>[2x]TNRDIQFTSFNGKDYPLCFLDEKTPLLFQWFERNPARFGKNDIPIINTEKNPYLNNIIKAATIEKERLIGIFVDGDFFPGQKDAFSKLEYDYENIKVIYRNDIDFSMYDKKLSEIYMENISKQESMPEEKRDCHLLQLLKKELSDIQEGNDSLIKSYLLDKGHGWADFYRNMAMLKAGQLFLEADKVGCYDLSTNSGCIYLDADMIITEKLGGIYIPDGIAVHVERIDGRASMENGIIAVDRNNHPALLAGLEIMHTKFDADPYSDGVCNGIRKHFNYSLNEDYNSFCDFIEFKHDNIIMNTSQ

Escherichia coli NleB1, Citrobacter rodentium NleB, and Salmonella enterica SseK1/3 type III effectors fatally glycosyltransfer N-acetyl glucosamine (GlcNAc) from UDP-GlcNAc to arginine residues of death domain-containing proteins that regulate host inflammation, intra-bacterial proteins, and themselves, whose post-translational modification disrupts host immune functions and prolongs bacterial viability inside host cells. All NleB/SseK orthologs have a typical GT-A conformation with two abutting β/α/β Rossmann domains unlike a GT-B consisting of facing each other β/α/β Rossmann domains with a flexible linkage and share a high degree of structural similarity. Several structural cores were revealed for the new arginine N-glycosylation systems: a catalytic DxD motif to position the Mn2+ cofactor and UDP-GlcNAc donor substrate, His-Glu-Asn (HEN) motif to select UDP-GlcNAc as a suitable donor substrate before other sugar donors such as UDP-Glc/Gal, C-terminal loop to stably embrace the UDP-GlcNAc donor substrate, and Helix-Loop-Helix (HLH) domain predicted to select the acceptor targets. The SseK1 effector GlcNAcylates Arg9, Arg190, Arg160, and Arg149 of four proteins involved in methylglyoxal detoxification, namely, GloA, GloB, GloC, and YajL, respectively, and catalyze methylglyoxal detoxification to significantly enhance their activity.

In all apo- and UDP-bound NleB1/SseK1/SseK3 effectors, the DxD motifs lie in the 219YLDADM224/221YLDADM226/224YLDADM229 regions and their quaternary DADM motifs form a Type-I-turn by H-bonding between the backbone CO(i) and NH(i + 3) groups, while the free Asp oxygen (Oδ of Asp221/Asp223/Asp/226) in the DxD motif interacts with the hydroxyl oxygen (Oη of Tyr219/Tyr221/Tyr224), named as a YD bond. In particular, apo NleB1/SseK1/SseK3 effectors have the free oxygen Oδ of the first catalytic aspartate in the DxD motif, ready to catch Mn2+ and UDP-GlcNAc. All N-glycosylated NleB/SseKs form a Type-I-turn in the DxD motif in the ligand-bound state, and the pathogenic NleB1/SseK1/3 toxins also retain Type-I-turn in the DxD motif in the apo state. Apo Clostridium toxin TcnA and apo E. coli NleB2 have twice intertwined Asx-β-turns, where Type-I-turns H-bond between the backbone CO of D284/D218 and the backbone NH of F287/M221, and the Asx-turn C10 H-bonds between the side chain of D284/D218 and NH of D286/D220 in apo TcnA/NleB2. These results indicate that the first catalytic aspartate in Apo TcdA/B, TcsL, SseK1/3, and NleB1 DxD motifs is open to bind Mn2+, whereas those of Apo TcnA, SseK2, and NleB2 are tightly tied by the second aspartate backbone in the Asx-turn of the DxD motif and are unable to bind Mn2+ and their ligand.(3R)-1-(2-fluorophenyl)-3-(methylamino)pyrrolidin-2-one 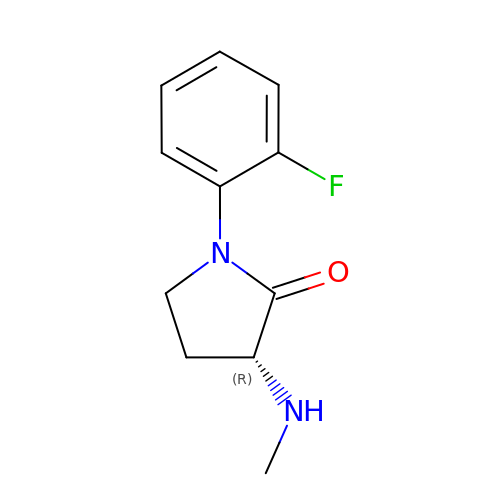| C11 H13 F N2 O | LXSCPIWTZCIAIQ-SECBINFHSA-N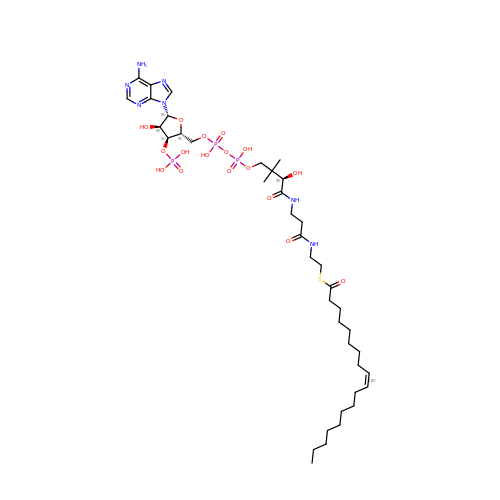S-{(3R,5R,9R)-1-[(2R,3S,4R,5R)-5-(6-amino-9H-purin-9-yl)-4-hydroxy-3-(phosphonooxy)tetrahydrofuran-2-yl]-3,5,9-trihydroxy-8,8-dimethyl-3,5-dioxido-10,14-dioxo-2,4,6-trioxa-11,15-diaza-3lambda~5~,5lambda~5~-diphosphaheptadecan-17-yl} (9Z)-octadec-9-enethioate (non-preferred name) | C39 H68 N7 O17 P3 S | XDUHQPOXLUAVEE-BPMMELMSSA-N> MAITTGTTEAQALNMTMRDAVLKVAPGVQQL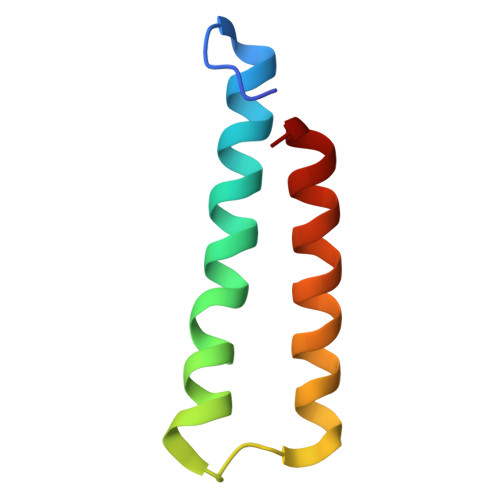VQNSSQLTAAEIAIIQTNITALKAAFTAAGA Neuronal nicotinic acetylcholine receptors (nAChRs) are ligand gated ion channels involved in the modulation of neurotransmission in the central and peripheral nervous system. α-Conotoxins are a large family of disulfide rich peptide antagonists of the nAChRs isolated from the venom of marine cone snails. Native LsIA is an equipotent antagonist of the human α7 and rat α3β2 but inactive at α3β4 nAChRs23 despite relatively high sequence identity to α-conotoxins with activity at the α3β4 nAChRs23242526272829303132. Using a co-crystal structure of LsIA and Lymnaea stagnalis acetylcholine binding protein (AChBP) to guide mutational studies, we identified that LsIA arginine at position 10 (R10) and asparagine at position 12 (N12) determined LsIA inactivity at α3β4.

The structure of the LsIA and Ls-AChBP complex was determined at 2.8 Å and solved using molecular replacement. The asymmetric unit contains one pentamer with LsIA bound to all five binding pockets. The diffraction data and electron density maps were well defined except for certain residues on flexible loops (mostly AChBP loop F) that were excluded from the final model. LsIA retains the typical α-conotoxin binding orientation with solvent exposed N- and C-termini oriented to the bottom and the top of the pocket respectively and the α-helical backbone buried into the binding pocket. The C loop of Ls-AChBP is displaced outward by a distance of 10.54 ± 0.20 Å as measured between the Cys 187 Cα atom in Ls-AChBP/LsIA and the HEPES-bound Ls-AChBP structure, similar to other α-conotoxin complexes. Pair-wise interactions of LsIA with AChBP consisted of a combination of conserved α-conotoxin interactions and several interactions unique to the LsIA/Ls-AChBP complex. Interestingly, LsIA R10 forms unique hydrogen bonds with AChBP Q55 (3.2 ± 0.11 Å) and Y164 (3.2 ± 0.26 Å) on the minus face of the ligand binding pocket. In addition to the interactions of the variable residues, unique interactions of LsIA N12 with Q73 (2.9 ± 0.05 Å), R104 (3.2 ± 0.07 Å) on the variable minus face(16,37) of the ligand binding pocket were also observed. Regardless, hydrogen bonds of LsIA N12 were consistently observed in all five binding pockets, suggesting an important role of this residue in LsIA activity. In the LsIA/Ls-AChBP co-crystal structure, LsIA N6 interacts with AChBP Y185, which is conserved across the nAChR subtypes and therefore not expected to influence subtype selectivity.

>LDRADILYNIRQTSRPDVIPTQRDRPVAVSVSLKFINILEVNEITNEVDVVFWQQTTWSDRTLAWNSSHSPDQVSVPISSLWVPDLAAYNAISKPEVLTPQLARVVSDGEVLYMPSIRQRFSCDVSGVDTESGATCRIKIGSWTHHSREISVDPTTENSDDSEYFSQYSRFEILDVTQKKNSVTYSCCPEAYEDVEVSLNFRKKGRSEIL[5x];>[5x]SGCCSNPACRVNNPNICX1-(propan-2-yl)-1H-benzimidazole-5-carboxylic acid | 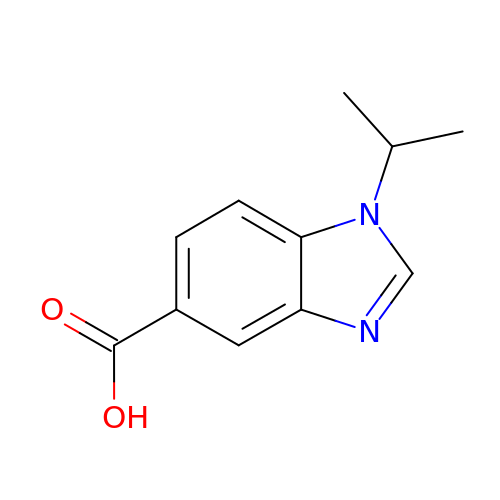C11 H12 N2 O2 | SQIQIYYPWAELAC-UHFFFAOYSA-N(2R)-2-({6-[BENZYL(METHYL)AMINO]-9-ISOPROPYL-9H-PURIN-2-YL}AMINO)BUTAN-1-OL | C20 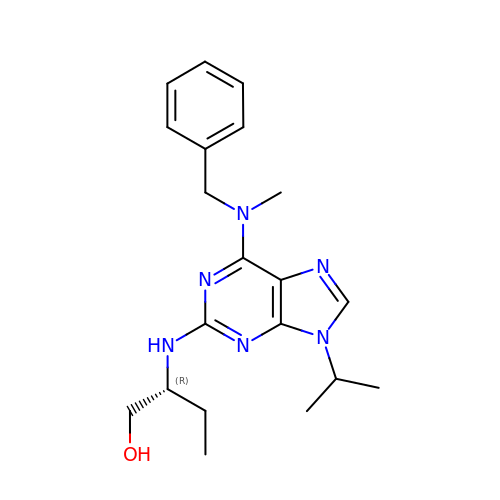H28 N6 O | YPYWONAECUVKHY-MRXNPFEDSA-N>[4x]TGLFVTLEGPEGAGKSTNRDYLAERLRERGIEVQLTREPGGTPLAERIRELLLAPSDEPMAADTELLLMFAARAQHLAGVIRPALARGAVVLCDRFTDATY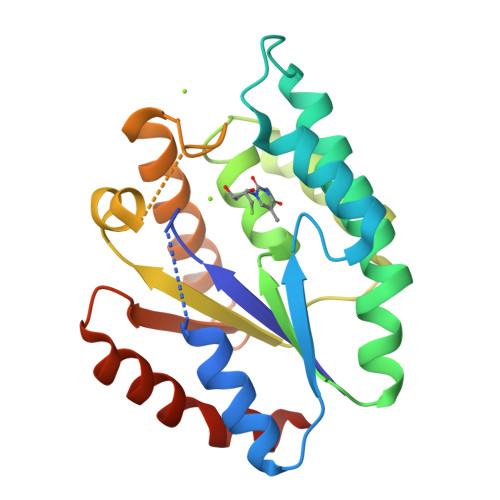AYQGGGRGLPEARIAALESFVQGDLRPDLTLVFDLPVEIGLARAAARGRLDRFEQEDRRFFEAVRQTYLQRAAQAPERYQVLDAGLPLAEVQAGLDRLLPNLLERLNGGS> VSIDYRHEMQDTAQAGHKDRLLISHRFANGFGLSSEVKWAQSSADKTPNKPFNEQVSNGTEVVASYVYKFNSVFSIEPGFSLESGSSNNNYRPYLRGRANVTDDLSVALRYRPYFKRNSGNIGKDNTMDKGYTLTGN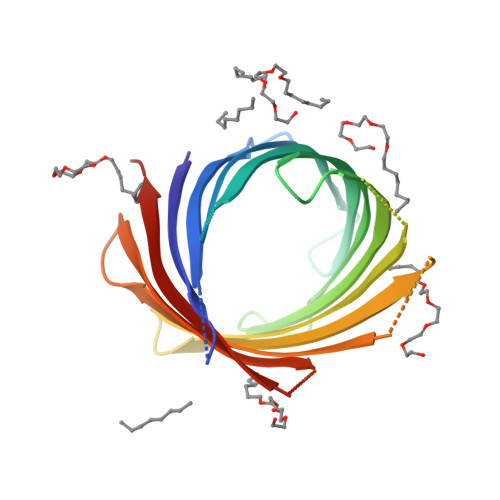IDYTFLKDYTIGYELEYKKGTSGKTILSDNDDYDITHNVKLSYKWDKNWKPYVEVGNVSGSETTDERQTRYRVGVQYSFHHHHHH N-(1-benzylpiperidin-4-yl)-4-iodobenzamide 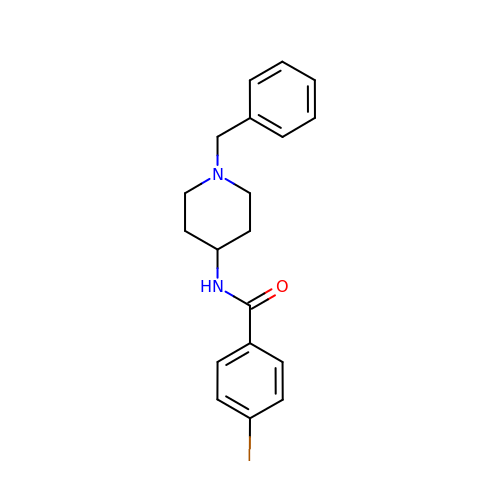| C19 H21 I N2 O | HELCSESNNDZLFM-UHFFFAOYSA-N>[2x]MGLQPPIHLFLVCFPAQGHINPMLRLAKRLAAKGLLITFSTTEHAGKDIRQANNIIDDQLTPVGNGFIRFEFFEDDCIEDDPKRRDLDFYVPQLELKGKEFLPETIKRHEKEGRPVFCFVNNPFIPW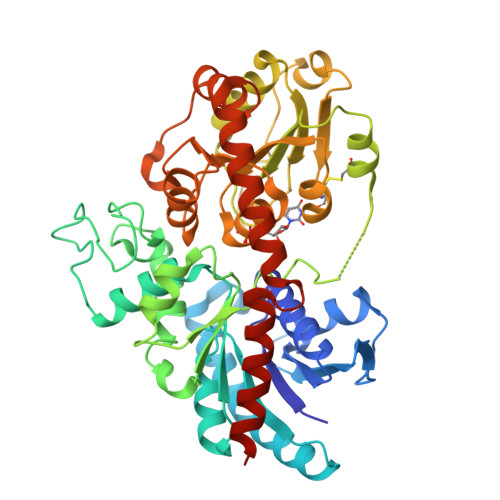VCDVAEDLGIPCATLWIQSCAVFSCYYHYFHKTVPFPSELDPSVDVQLPNLPLLEYDEIPSFLHPSSPYKILGTAILGQFKNLSKSFCVLADTFDELEHEIIEGMSKFCKVKTVGPLFKNPKASVSNIRGDMLKADDCLDWLDSKSPGSVVYISFGTIAYIKQEQVEEIAYGLLNSGVSFLWVMKPPDVAFGYDLHVLPDGFMEKIGTRGKIVQWCPQEQVLAHPSVACFLTHCGWNSTVEALTSGVPVLAYPQWGDQVTNAKFLVDVYGVGVRLCRGEAENKVIPRDVIGKALVEATVGKRAVELKENATRWKKAAEEAVAEGGSSDRNIQDFVEEIRKRSGLYNSKPAAT>[2x]GHMSARVRPFLMFQ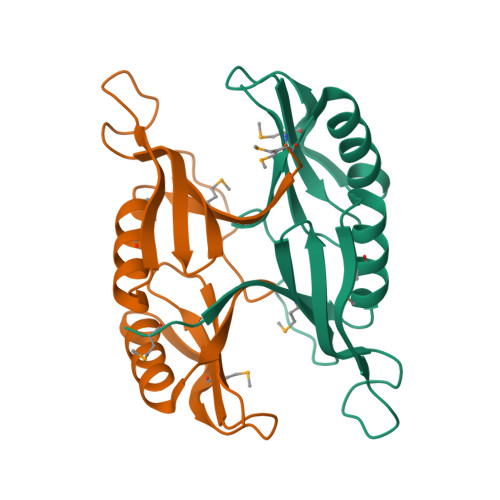GVQAEAAMNFYLSLFDDAEILQIQRYGAEGPGPEGSVLKALFRLGDQSVHCIDSHVRHAFDFTPAFSFFVDCESNAQIERLAEALSDGGKALMPLGDYGFSQRFAWLADRFGVSWQLNLAGS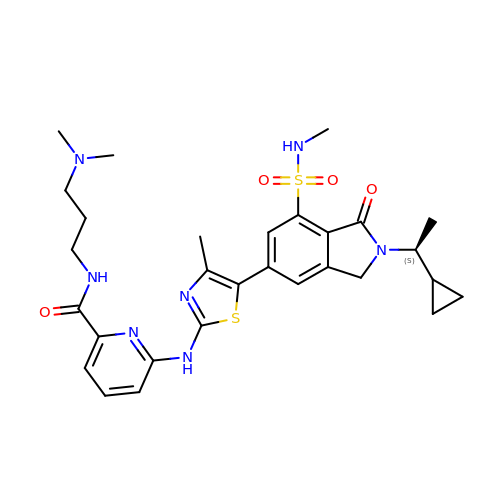6-[[5-[2-[(1S)-1-cyclopropylethyl]-7-(methylsulfamoyl)-1-oxidanylidene-3H-isoindol-5-yl]-4-methyl-1,3-thiazol-2-yl]amino]-N-[3-(dimethylamino)propyl]pyridine-2-carboxamide | C29 H37 N7 O4 S2 | SMMGDTUHUMCVSB-SFHVURJKSA-N>[2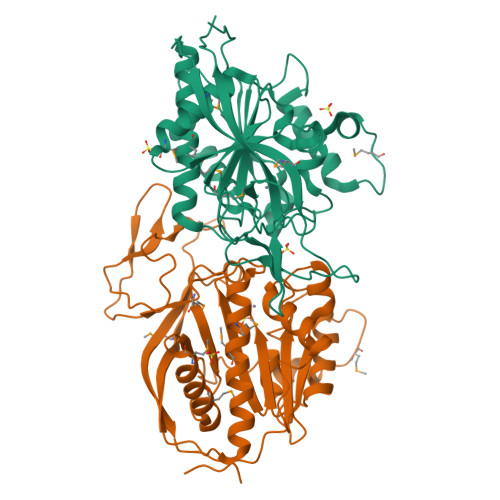x]STSCVAEEPIKKIAIFGGTHGNELTGVFLVTHWLKNGAEVHRAGLEVKPFITNPRAVEKCTRYIDCDLNRVFDLENLSKEMSEDLPYEVRRAQEINHLFGPKNSDDAYDVVFDLHNTTSNMGCTLILGDSGNDFLIQMFHYIKTCMAPLPCSVYLIEHPSLKYATTRSIAKYPVGIEVGPQPHGVLRADILDQMRRMLKHALDFIQRFNEGKEFPPCAIDVYKIMEKVDYPRNESGDVAAVIHPNLQDQDWKPLHPGDPVFVSLDGKVIPLGGDCTVYPVFVNEAAYYEKKEAFAKTTKLTLNAKSIRSTLH> MERMNWLSRLASRGPGHRIPQGANLQTPVMADPETCLMVFKNHWSQVVRILERQGPRAAPGGADDLSAVRNHTYQMLTLLAEDRAVPSAPTGPGPLLEFALHEDLLTRVLTWQLQWDELGDGVEERRAEQLKLFEMLVSEARQPLLRHGPVREALLTLLDACGRPVPSSPALDEGLVLLLSQLCVCVAQEPSLLEFFLQPPPEPGAAPRLLLFSRLVPFVHLEGTLGQQARDALLLLMALSAGSPTVGRYIADHSYFCPVLATGLSALYSSLPRKIEVPGDDWHCLRREDWLGVPALALFMSSLEFCNAVIQVAHPLVQKQLVDYIHNGFLVPVMGPALHKTSVEEMIASTAYLELFLRSISEPALLRTFLRFLLLHRHDTHTILDTLVARIGSNSRLCMVSLSLFRTLLNLSCEDVLLQLVLRYLVPCNHVMLSQKPAVRDVDLYGRAADKFLSLIPRCCRHHAPSPPRPEHASWARGPGSPSVDSSSVTTVPRPSTPSRLALFLRQQSLGGSESPGPAPCSPGLSASPASSPGRRPTPAEEPGELEDNYLEYLREARRGVDRCVRACRTWSAPYDGERPSPEPS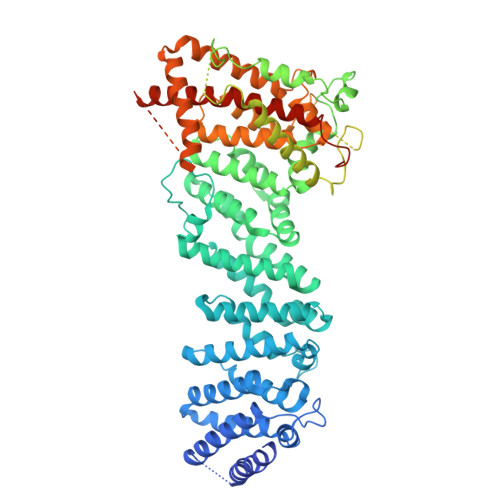PFGSRTKKRSLLPEEDRNNVGEGEEEELGRRGRAGGAGEGPGHLPPPQLNGVPGSWPEGAKKVRLVPKEGAGELLEGISEGMAGLEGFGQELRELEVALSNGGTGSESPLEPPLPLEEEEAYESFTCPPEPPGPFLSSPLRTLNQLPSQPFTGPFMAVLFAKLENMLQNSVYVNFLLTGLVAQLACHPQPLLRSFLLNTNMVFQPSVKSLLQVLGSVKNKIENFAASQEDFPALLSKAKKYLIARGKLDWAEGPAAGPAPRRSDPLVKSRRPSLGELLLRHAHSPTRARQAAQLVLQPGRDGAGLGLSGGSPGASTPVLLTRGGAPERQGEALRVKNAVYCAVIFPEFLKELAAISQAHAVTSPFLLETSEEGSGPLISGCGPLNP(3S,5R)-5-[4-(2-chlorophenyl)-2,2-dimethyl-5-oxopiperazin-1-yl]-N-(3-methylbutyl)piperidine-3-carboxamide 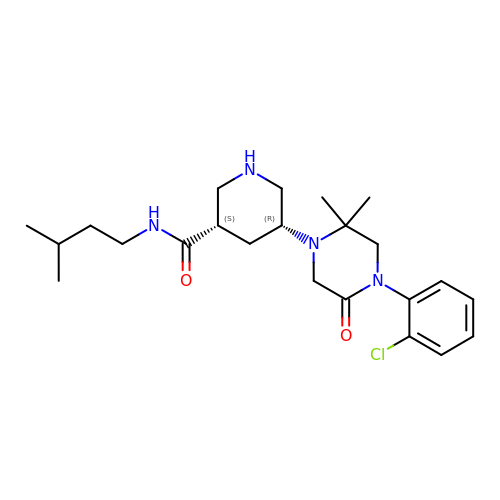| C23 H35 Cl N4 O2 | OIPASSZLGANZOF-ZWKOTPCHSA-N>[2x]FNILLATDSYKVTHYKQYPPNTSKVYSYFECREKKTENSKLRKVKYEETVFYGLQYILNKYLKGKVVTKEKIQEAKDVYKEHFQDDVFNEKGWNYILEKYDGHL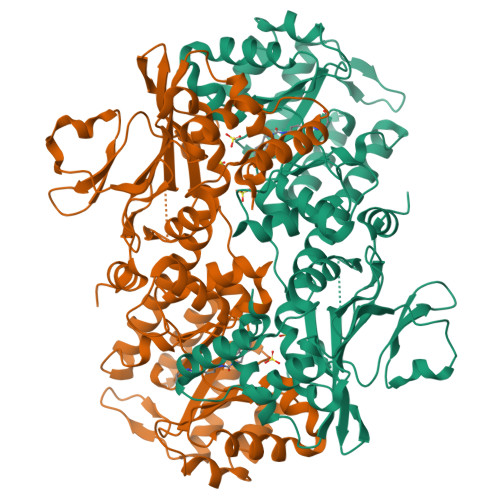PIEIKAVPEGFVIPRGNVLFTVENTDPECYWLTNWIETILVQSWYPITVATNSREQKKILAKYLLETSGNLDGLEYKLHDFGYRGVSSQETAGIGASAHLVNFKGTDTVAGLALIKKYYGTKDPVPGYSVPAAEHSTITAWGKDHEKDAFEHIVTQFSSVPVSVVSDSYDIYNACEKIWGEDLRHLIVSRSTQAPLIIRPDSGNPLDTVLKVLEILGKKFPVTENSKGYKLLPPYLRVIQGDGVDINTLQEIVEGMKQKMWSIENIAFGSGGGLLQKLTRDLLNCSFKCSYVVTNGLGINVFKDPVADPNKRSKKGRLSLHRTPAGNFVTLEEGKGDLEEYGQDLLHTVFKNGKVTKSYSFDEIRKNAQLNIE>MGHHHHHHMLENIRDAVRKFLTGSTPYEKAVDEFIKDLQKSLISSDVNVKLVFSLTAKIKERLNKEKPPSVLERKEWFISIVYDELSKLFGGDKEPNVNPTKLPFIIMLVGVQGSGKTTTAGKLAYFYKKRGYKVGLVAADVYRPAAYDQLLQLGNQIGVQVYGEPNNQNPIEIAKKGVDIFVKNKMDIIIVDTAGRHGYGEETKLLEEMKEMYDVLKPDDVILVIDASIGQKAYDLASRFHQASPIGSVIITKMDGTAKGGGALSAVVATGATIKFIGTGEKIDELETFNAKRFVSRILGMGDIESILEKV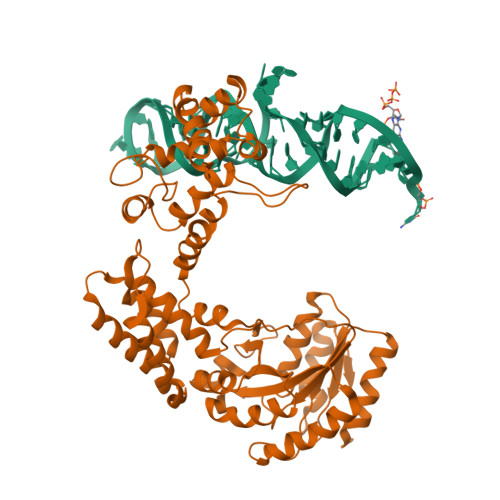KGLEEYDKIQKKMEDVMEGKGKLTLRDVYAQIIALRKMGPLSKVLQHIPGLGIMLPTPSEDQLKIGEEKIRRWLAALNSMTYKELENPNIIDKSRMRRIAEGSGLEVEEVRELLEWYNNMNRLLKMVK[4x]> MKDLSHYGPALCVKFYNDYVLAGYGPFIHVYDYHSATLINKCRLFHYNKVHGLSLSSEGKILAYGARSVTIVELEDVLKKESLVDFERINSDWITGATFSFDNLQIYLLTCYNKVLICDLNCEVLFRKSLGGERSILYSGIIKVFGPDKVYVNAGTVMGGVIIWDLFSETKIHNLLGHEGSIFYVNLSNNGRYVASCSDDRSIRLWDLETGKQLSVGWSHTARIWNLMFFDNDSKLISVSEDCTCRVWNIIESRENVAELSISNVYEVHLIKSIWGVDVKDDEMIAVTSGNDGRLKLIDLLQLKRHGDEETSFSLDDIAKQCGDIFEKNESIKGFQWFSFGVIAITSLGKILKYSDVTKQWKLLLTNEKFNSYPITNGIQTQNIAVFSNNKSDILLIKFSKDSADIIETEEFHLDELSKTNNCLVTEYDDDSFLLTLQSPNPREKFVCLEISLQNLKIKSKHCFNKPENFSSSCLTSFRNHILVGSRFSTLVIYNLLDESEEPFIIRRLSPGDTTTSIEFVEDKDNSAVFSVTNRDGYYVFIELTKNSLEEGPYRLSYKVLHSNKMMKGFLEGAFFNSKGEYITYGFKSSLFY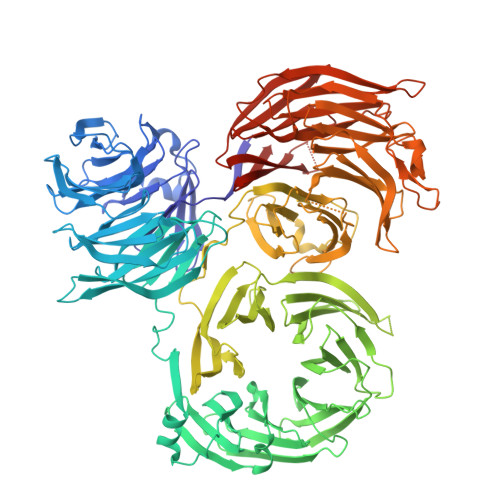LYNETNCYELASEVCGGSHRLWNLAKITDGHVLMYIKASRFHLRKIYNSIVPETLENGVHGREIRDISICPVSNTNTNDNFKDGHIFCTASEDTTIKLGYFNNRTGKVQNFWTQRKHVSGLQRCQFINHKLMISSSAREELFLWELNDKYNKRPYMTIRQALPVSTNNSDLRIMDFDVKFISQSGDFLLVTVYSDSTIKIWHYRENQNKFDLIMQGRYKTCCLFNVVFIALKEELLVVISPTDGHLVVYNITEYVPFSVDPISGDLVDHKLDATISNLPAPVAQLPVHQSGVKSLDYVANATRTSATILTGGDDNGLGLSNLKLDDSNKVTLKTSDFIAAAASSTITSGMLINGGKEVITTSVDQVIRAWEITAGKLSLVDKKRTTVADTGSLEIISNDEDADSEKTLLIGGVGLSIWKKLEVLFQGPSHHHHHH>MAHHHHHHVGTSSNLSFEHTDNILIEERLFPPPEDIVKNANITAYMKSKGFDDYEAFYRWSLANRFEFWNDMAKELHWFEPWKSTFEWTDKPFFKWFTDGKFNIAYNCLDRYMGTPIEDKVAFYWEGDDGSSRAYTYKEMYVLTNRVAKVLQNQGVKKGDRVAIYMPMIPEMAASVLACARLGAPHMVVFGGFAASSLRDRMNDCDAKVLITADGGYRGGKVIELKKIADEAVAETPTIEKVFVQRHTGFEVPMAEGRDVYLDVLLNDIPEDTVVPCEPVDSEDMLYILYTSGSTGKPKGVVHVHGGYAVGCYATTKFVFDIKPSDVFWCTADIGWVTGHSYTIYGPMMNAASIVLFEGIPTYPAADRFWSIVEKYKVNIIYTAPTAIRSLMRFGEELPARHDLSSLRILGTVGEPINPEAWMWYRKNIGHNELPIMDTWWQTETGMILISPTPILPLKPGSASRPLPTIEADVVNKDGKPVGPEHGGFLIIRHPWPAQMRTIFGDPDRYKTYWETIPDVYFAGDAATMDKMGYFRIQGRVDDVIKVSGHRLGSMEIESSLVSHPAVAEAAAIGKPDEVKGEHVKVFVILRNGVEPTESLAVELKRHVRTLVGPLATPDELEFVTSLPKTRSGKIMRRVVRARELGEPVGDITTLDV[4x]

The AMP-forming acetyl-CoA synthetase is regulated by lysine acetylation both in bacteria and eukaryotes. AMP-forming acetyl-CoA synthetases catalyse the ATP-dependent formation of acetyl-CoA from acetate and coenzyme A in two half-reactions. In the first half-reaction, acetyl-CoA synthetase activates acetate using ATP to form acetyl-AMP under the release of pyrophosphate PPi (adenylation reaction). In the second half-reaction, the thioester acetyl-CoA is generated from the mixed anhydride acetyl-AMP and CoA releasing AMP (thioesterification/thioester-formation).

Crystal structures of AcsA from Chloroflexota bacterium in the apo form and in complex with acetyl-adenosine-5′-monophosphate (acetyl-AMP) support the flexible C-terminal domain adopting different conformations. Several structures were available for AMP-forming enzymes in their apo states and in complexes with various ligands suggesting that these enzymes can exist in at least three states (apo forms with flexible conformations of the C-terminal domain, CoA/acyl-AMP, AMP/ATP/substrate form). Ligand binding stabilizes the C-terminal domain in the conformations to catalyse the first or second half-reaction, and without ligands, the C-terminal is flexible and can adapt to different conformations. Notably, we found in the apo structure and in the acetyl-AMP-bound AcsA structure of the Chloroflexota bacterium a phosphorylated histidine residue, i.e. His476, in the C-terminal domain. This histidine is not conserved amongst other members of AMP-forming acetyl-CoA synthetases. Although the Chloroflexota bacterium AcsA is a monomer in the crystal structure (supported by PISA server) and analytical SEC supports the monomeric form in solution, we observed in the crystal structure that two trimers (a crystallographic as well as a non-crystallographic trimer) are formed with an app. 500 Å2 buried surface area between neighbouring molecules, with the phospho-His476 close to the threefold rotation axes. Whether this is relevant for a physiologically important process, such as oligomerisation, needs further validation.>MRLTKFTDLALRSL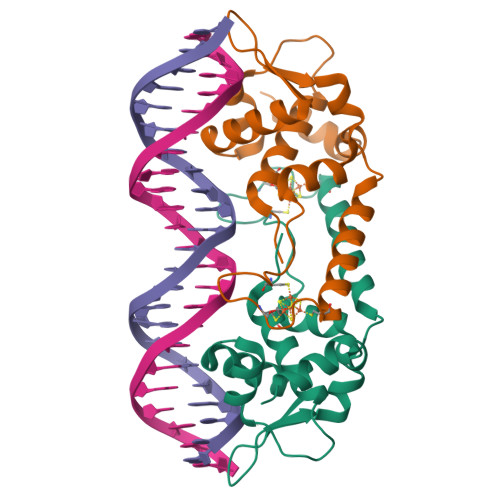MRLAVVRDGDEPLATREVAEVVGVPYTHAAKAITRLQHLGVVEARRGRGGGLTLTDLGRRVSVGWLVRELEGEAEVVDCEGDNPCPLRGACRLRRALRDAQEAFYAALDPLTVTDLVAAPTGPVLLGLTDRPSGKLAAALEHHHHHH[2x]>[2x]GPNPYDRKRQDKAPVGLKNVGNTCWFSAVIQSLFNLLEFRRLVLNYKPPSNAQDLPRNQKEHRNLPFMRELRYLFALLVGTKRKYVDPSRAVEILKDAFKSNDSQQQDVSEFTHKLLDWLEDAFQMKAEEETDEEKPKNPMVELFYGRFLAVGVLEGKKFENTEMFGQYPLQVNGFKDLHECLEAAMIEGEIESLHSENSGKSGQEHWFTELPPVLTFELSRFEFNQALGRPEKIHNKLEFPQVLYLDRYMHRNREITRIKRE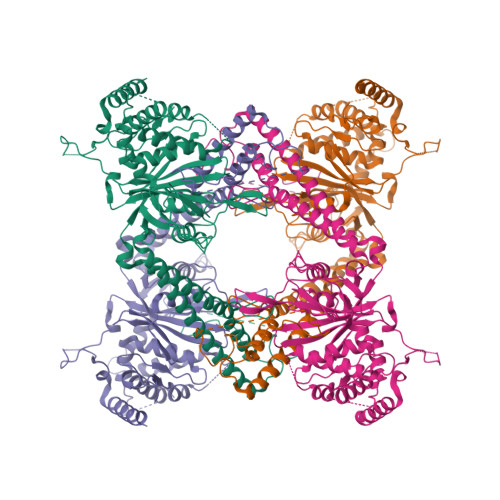EIKRLKDYLTVLQQRLERYLSYGSGPKRFPLVDVLQYALEFASSKPVCTSPVDDIDASSPPSGSIPSQTLPSTTEQQGALSSELPSTSPSSVAAISSRSVIHKPFTQSRIPPDLPMHPAPRHITEEELSVLESCLHRWRTEIENDTRDLQESISRIHRTIELMYSDKSMIQVPYRLHAVLVHEGQANAGHYWAYIFDHRESRWMKYNDIAVTKSSWEELVRDSFGGYRNASAYCLMYINDKAQFLIQEEFNKETGQPLVGIETLPPDLRDFVEEDNQRFEKELEEWDAQLAQKALQE> VAHFTFQPDPEPREYGQTQKMNLFQSVTSALDNSLAKDPTAVIFGEDVAFGGVFRCTVGLRDKYGKDRVFNTPLCEQGIVG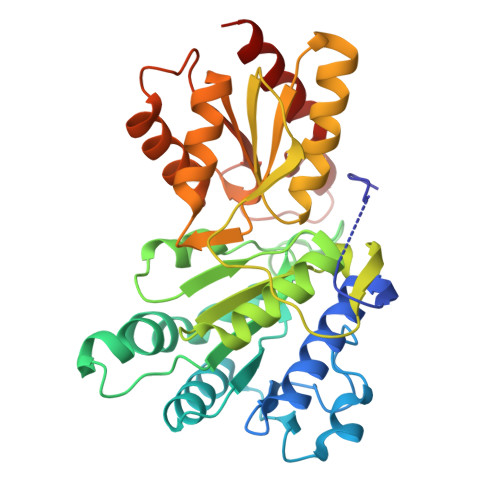FGIGIAVTGATAIAEIQFADYIFPAFDQIVNEAAKYRYRSGDLFNCGSLTIRSPWGCVGHGALYASQSPEAFFAHCPGIKVVIPRSPFQAKGLLLSCIEDKNPCIFFEPKILYRAAAEEVPIEPYNIPLSQAEVIQEGSDVTLVAWGTQVHVIREVASMAKEKLGVSCEVIDLRTIIPWDVDTICKSVIKTGRLLISHEAPLTGGFASEISSTVQEECFLNLEAPISRVCGYDTPFPHIFEPFYIPDKWKCYDALRKMINY>ALLPILSFPDPRLRTIAKPVEEVTDEIRQLAADMFETMYAAPGIGLAASQVDRHIQLIVMDLSESKDEPMVFINPKVTPLTEETQPYEEGCLSVPQIYDKVDRPSRVKIEAINLEGQAFEIEADGLLAVCIQHEMDHLNGKLFVDYLSPLKRQRAREK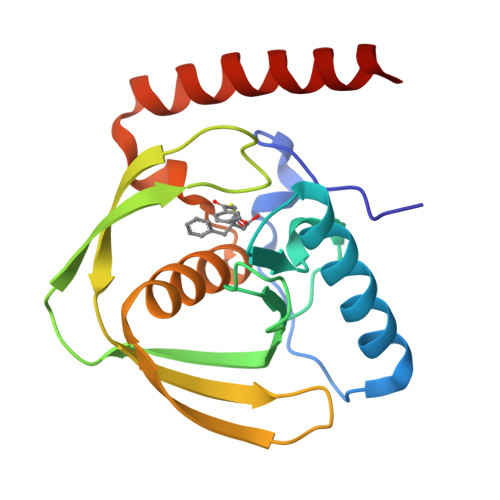VEKIVRQREREK[2x]>[3x]SLGSL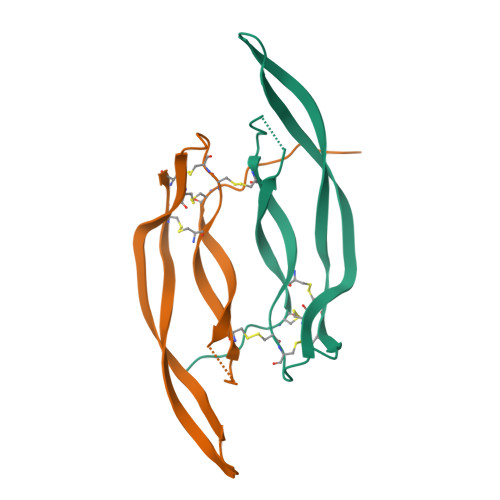TIAEPAMIAECKTRTEVFEISRRLIDRTNANFLVWPPCVEVQRCSGCCNNRNVQCRPTQVQLRPVQVRKIEIVRKKPIFKKATVTLEDHLACKCETVAAARPVT N-methyl-4-sulfamoylbenzamide | C8 H10 N2 O3 S | 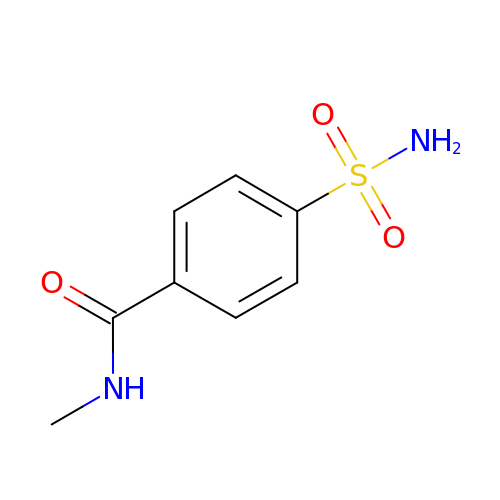CTDFBRMMEMHBEO-UHFFFAOYSA-N>AAKTEQQIADIVNRTITPLMQEQAIPGMAVAVIYQGKPYYFTWGKADIANNHPVTQQTLFELGSVSKTFNGVLGGDAIARGEIKLSDPVTKYWPELTGKQWQGIRLLHLATYTAGGLPLQIPDDVRDKAALLHFYQNWQPQWTPGAKRLYANSSIGLFGALAVKPSGMSYEEAMTRRVLQPLKLAHTWITVPQNEQKDYAWGYREGKPVHVSPGQLDAEAHGVKSSVIDMARWVQANMDASHVQEKTLQQGIALAQSRYWRIGDMYQGLGWEMLNWPLKADSIINGSDSKVALAALPAVEVNPPAPAVKASWVHKTGSTGGFGSYVAFVPEKNLGIVMLANKSYPNPVRVEAAWRILEKLQ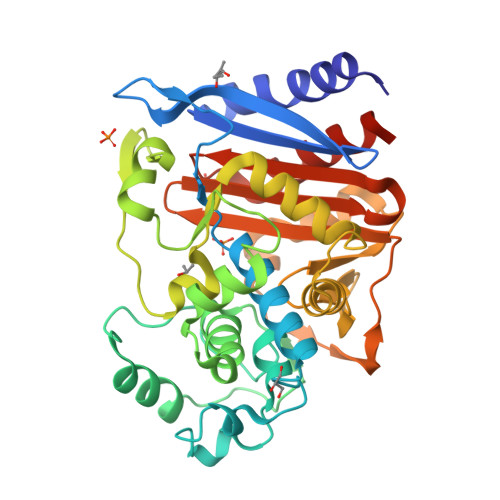FEHHHHHHHH[2x]> MTTRTKGRGHTVATTQNDRMPGPELSGWISEQLMTGRIPVNDIFCDIENNPGLCYASQMQQTKPNPKMRNSQTQTDPICNHSFEEVVQTLASLATVVQQQTIASE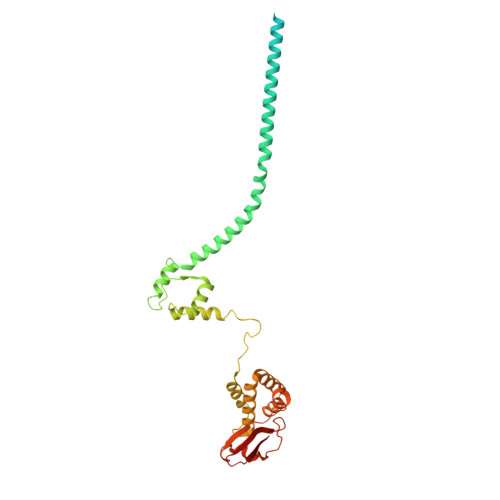SLEQRITSLENGLKPVYDMAKTISSLNRVCAEMVAKYDLLVMTTGRATATAAATEAYWAEHGQPPPGPSLYEESAIRGKIESRDETVPQSVREAFNNLDSTTSLTEENFGKPDISAKDLRNIMYDHLPGFGTAFHQLVQVICKLGKDSNSLDIIHAEFQASLAEGDSPQCALIQITKRVPIFQDAAPPVIHIRSRGDIPRACQKSLRPVPPSPKIDRGWVCVFQLQDGKTLGLKI>[4x]MPTRAAVTVKPDDHRYDLLARADNYRFVAQPEYFRLPYSTAQVVEAVSEAVAAGKRLTVRSGGHCGEAFVASPDVDVIVDLSSMSHVGYDEERGAFEVEAGATVGQIYRVLYKNYGVTFPGGFCMGVGAGGHISGGGYGPLSRLLGLTVDYLHAVEVVVVDAEGVVST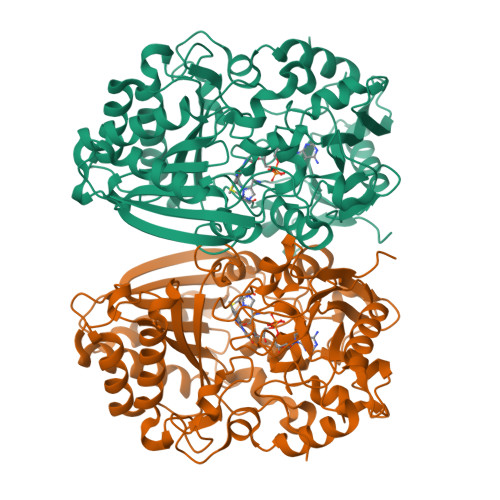VVATREEDDPNRDLWWAHTGGGGGNFGVITRYWLRSPDAVGDAPEEALPRPPASFHVARVSWSWAELTEADYVRLVSNFLDWQLRNCTVDSPNIGLYALLECFHRSAGHLAMHAQIPVDVPDAEERMSWFLAELNEGVAVAPSLTRRRLPWLATSQLLAIPDVGPGAIGVRRKVKSADLRGPHTREQLAAAYRHLSRADYHCPSAAMEYIAYGGRVNTVDPAATAVPRGASLKTFYMVAWTDPDEDEEHLRWIREIYRDIHSATGGVPTPDEVNTGAYINYPDIDLADPEWNTSGVPWHTIYYGDNYPRLQEIKSRWDPRNVFRHAFSIRPR> Q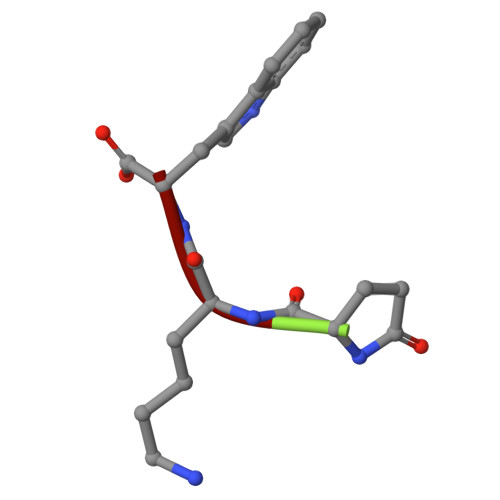KW> MRSEVKIGLALTALLVAVTAAGAASIKNTKHDLSSGSTGATFKATN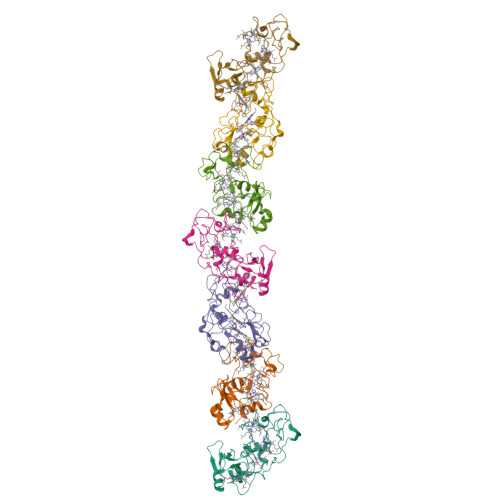TDQICVFCHTPHNAQQDIPLWNRGNPTASTFTLYSSSSMNNVPVKQGFTADSISLFCMSCHDGATGLGGAVHNDPNGAAIAMVGGNDLITGEANLGTDLSNDHPVNFEVTPAGIAADGNLGALDTGTNPPTMKTGDVTNGLPLFKSARGATTLECGSCHKVHDNTDAPFLRTTMAGSKLCLGCHKK> MDEGMWLMQQLGRKYAQMKERGLKMKEYDLYNPNGTSLKDAVVLFDGGCTGEVVSDRGLVLTNHHCGYDMIQAHSTLEHNYLENGFWAMREADELPNKDISVVFIDKIEDVTDYVKKELKAIKDPNSMDYLSPKYLQKLADKKAGKNFSAKNPGLSVEIKAFYGGNLYLMFTKKTYTDVRLVGAPPSSIGKFGADTDNWIWPRHTGDFSIFRIYADKNGNPAPYSEDNVPLKPKRFFNISLGGVQE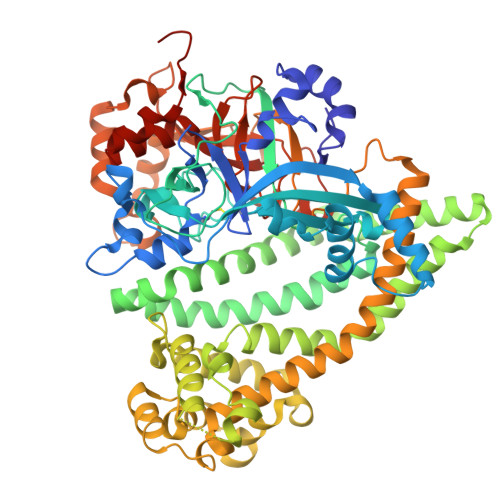NDYAMIMGFPGTTHRYFTASEVDEWKSIDNDIRIRMRDIRQGVMLREMLADPQIKIMYSAKYAASQNAYKRAIGANWAIKTRGLRQNKQAMQDRLIAWGAKQGTPRYEEAVHEIDATVAKRADLRRRYWMIEEGIIRGIEFARSPIPTEDETKALQGNDASARKEAIDKIRTRYSKFANKDYSAEVDKKVAVAMLTEYLKEIPYENLPLHLRLVKDRFAGDVQAYVDDIFARSVFGSEAQFDAFAAVPSVEKLAEDPMVLFASSVFDEYRKLYNELRPYDDPILRAQRTYIAGLLEMDGDQDQFPDANLTLRFTYGQVKGYSPRDNVYYGHQTTLDGVMEKEDPDNWEFVVDPKLKAVYERKDFGRYADRSGRMPVAFCATTHTTGGNSGSPVMNANGELIGLNFDRNWEGVGGDIQYLADYQRSIIVDIRYVLLVIDKVGGCQRLLDEMNIVPAHHHHHH>[4x]MVKVDLESKRYGEKLKEVFLMLDNNVVECIKEITESSRNGKLVFFVGAGVSTLSDYPQWWRLVDKYHEELYGSPKKGNYSSDEYLRIPQIFYNVKGEMAFDGILKDFFQVDKPTNPIHDKILAMNPAHVITTNYDNLIDTACWKRGKYFSVISAEEDVANATSSRYLLKVHGDFRKGFKGENVVLKEDDYLNYDQNYPLISNLMKTIIATHTIVFIGYGLGDYNINMLLNWVRKLQKDSFHKPFFIRTDPSPIENETLIYYENKGLRIIDAASLIDSNEYDYLERYSAVMDLLIESQENKFITKDDEVIDYIYGKISPLFALQYIRKIDLKHVFEYDYHFEVNGTVVRHKNKGFGYMERFFELKESCDERSKLSKKQYERFNALFNFFEKNGVICMAKDAGTLNTSIEINSLAYHGKYDVMKKFIEEQSVSIEDDYKKAFFLACLGRWEESYDLYSNIILNSIDESNGCVYYLSQINRYRIYQSITQAVTQFNGLGLLTFGRHYKPFTDEFLARIEREMTNFNIDDLFNGMPFEFQKKYKILEFLSDNQFLYDDTVKLFELTNKVRSEMSEGSYSFGMSSDIVVLLRLYDNLRFLYENCLWSVSFHEFHQYIRNSMSLLIEKAEYERTRDIDELGFSFFGKKSGFFMEYYDFVNISRHFKIDDIKNLERSCSIDKIRFGEQEKIEEYLVGIAEEITKQFSANGMNVVFYTQFISEAKAALYFAKYVKLSEEGLGKIVKALLFYFPERDLDIGKRYVWLERLTKCNELPKSIISIIDDFLVLQAEKHIDQNYSEVSSNGLYSRDYGALIKHFEKNFISKRLSEITLCLTQDKQKQIDFLFKLLPLLSTNAKSHLLSFKSVENINDLMNGIRIGLIDEFTPEHEELIIEYLETRKVNYIVEKEKGIQTFSSNDYMSTFGIWYFLEEINNSKMEEFIGMDDQYDFFVDPENFDYKKFIPSWLKNYNDKLLGKIAGNKHMKHHVIEVLKERVKNSNDKRYLEILMNYFI;>[2x]MIEIFKDTGATHDLVYHSKINTFVWDVEFDIVLSDSKELNKCYFVKCFNPYRINGKCDFAVSSIDIFSEGKRLLIENEFNFKITKAVHVATSKDVTEIVLHLSERISSPFPIVKEVVYLD

The defense-associated sirtuin 2 (DSR2) effector, a SIR2 domain-containing protein, protects bacteria from phage infection by depleting NAD+, while an anti-DSR2 protein (DSR anti-defense 1, DSAD1) is employed by some phages to evade this host defense. The NADase activity of DSR2 is unleashed by recognizing the phage tail tube protein (TTP). DSR2 is arranged as a dimer of dimers, which is facilitated by the tetramerization of SIR2 domains. DSR2 has a two-domain architecture, with the CTD responsible for sensing the infection signal and SIR2 acting to prevent phage propagation.

We therefore reconstituted the DSR2-DSAD1 binary complex and determined the cryo-EM structures at resolutions of 3.4–3.6 Å. We modeled four DSR2 molecules and two DSAD1 molecules into the EM density. The tetrameric DSR2 displays an elongated shape, with two DSR2 dimers forming a head-to-head tetramer (the four molecules are termed A, B, A’, and B’, respectively). Although each DSR2 dimer binds to one DSAD1 molecule, two binding modes are found in the context of the DSR2 tetramer. The second binding mode involves DSR2-A and DSR2-B’ molecules. However, these DSR2-DSAD1 trimeric subcomplexes in the two states are nearly identical. DSAD1 is trapped by the tip of the CTD fishhook. The H4 subdomain, along with the H3 subdomain from the adjacent molecule, brackets the β-hairpin of DSAD1. Notably, Tyr16 of DSAD1 stacks against Tyr574 and Phe576 from the adjacent H3 subdomain. The H4 subdomain moves outward by ~10 Å to accommodate DSAD1.>APQQINDIVHRTITPLIEQQKIPGMAVAVIYQGKPYYFTWGYADIAKKQPVTQQTLFELGSVSKTFTGVLGGDAIARGEIKLSDPTTKYWPELTAKQWNGITLLHLATYTAGGLPLQVPDEVKSSSDLLRFYQNWQPAWAPGTQRLYAGSSIGLFGALAVKPSGLSFEQAMQTRVFQPLKLNHTWINVPPAEEKNYAWGYREGKAVHVSPGALDAEAYGVKSTIEDMARWVQSNLKPLDINEKTLQQGIQLAQSRYWQTGDMYQGLGWEMLDWPVNPDSIINGSDN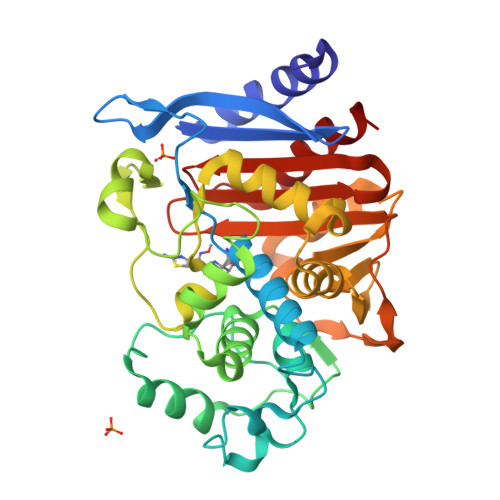KIALAARPVKAITPPTPAVRASWVHKTGATGGFGSYVAFIPEKELGIVMLANKNYPNPARVDAAWQILNALQ[4x]> MKKSKSKKKAAKAQEVEVKEPVKEPEPLPELEAAEDLQDLPEPDPELLASEPELEDLADPLDLEGPLEADLLPEEGLLEEEEEELSLPKVSTSDPVRQYLHEIGQVPLLTLEEEIDLARKVEEGMEAIKKLSEATGLDQELIREVVRAKILGTARIQKIPGLKEKPDPKT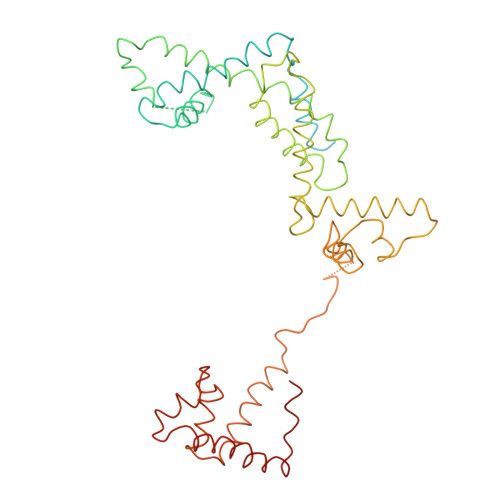VEEVDGKLKSLPKELKRYLHIAREGEAARQHLIEANLRLVVSIAKKYTGRGLSFLDLIQEGNQGLIRAVEKFEYKRRFKFSTYATWWIRQAINRAIADQARTIRIPVHMVETINKLSRTARQLQQELGREPSYEEIAEAMGPGWDAKRVEETLKIAQEPVSLETPIGDEKDSFYGDFIPDENLPSPVEAAAQSLLSEELEKALSKLSEREAMVLKLRKGLIDGREHTLEEVGAYFGVTRERIRQIENKALRKLKYHESRTRKLRDFLE>MKLIWSEESWDDYLYWQETDKRIVKKINELIKDTRRTPFEGKGKPEPLKHNLSGFWSRRITEEHRLVY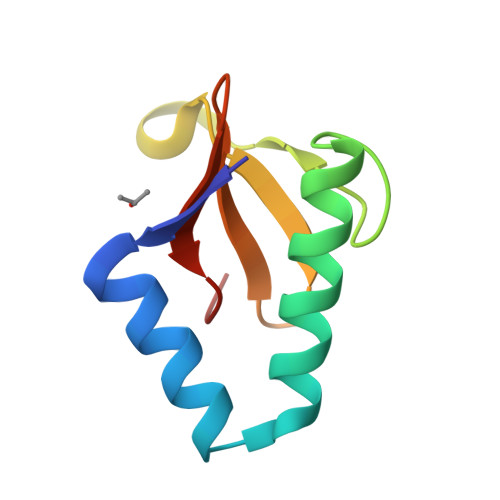AVTDDSLLIAACRYHY[4x]> KSCPNPGQIRNGQIDVPG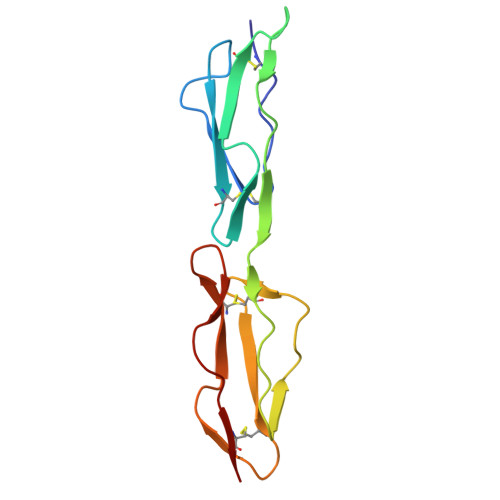GILFGATISFSCNTGYKLFGSTSSFCLISGSSVQWSDPLPECREIYCPAPPQIDNGIIQGERDHYGYRQSVTYACNKGFTMIGEHSIYCTVNNDEGEWSGPPPECRG> GAMGSMPHRTIHLFRKGLRLHDNPTLLAALESSETIYPVYVLDRRFLASAMHIGALRWHFLLQSLEDLHKNLSRLGARLLVIQGEYESVLRDHVQKWNITQVTLDAEMEPFYKEMEANIRRLGAELGFEVLSRVGHSLYDTKRILDLNGGSPPLTYKRFLHILSQLGDPEVPVRNLTAEDFQRCMSPEPGLAERYRVPVPADLEIPPQSLSPWTGGETEGLRRLEQHLTDQGWVANFTKPRTIPNSLLPSTTGLSPYFSMGCLSVRTFFQRL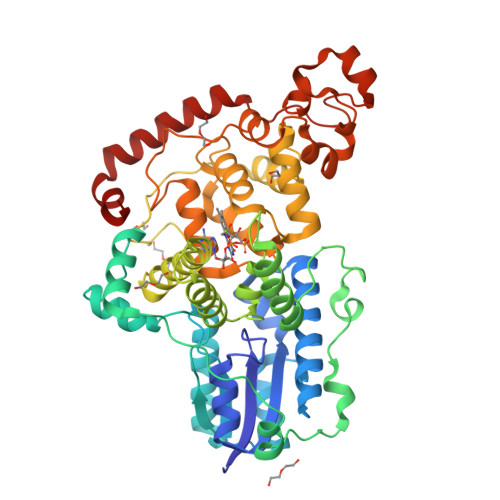SNIYAQAKHHSLPPVSLQGQLLWREFFYTVASATQNFTQMAGNPICLQIHWDEDAERLHKWKTAQTGFPWIDAIMTQLRQEGWIHHLARHAVACFLTRGDLWISWEEGMKVFEELLLDADYSINAGNWMWLSASAFFHHYTRIFCPVRFGKRTDPEGQYIRKYLPVLKNFPTKYIYEPWTASEEEQRQAGCIIGRDYPFPMVNHKEASDRNLQLMRRVREEQRGTAQLTR> AIGPVADLTISNGAVSPDGFSRQAILVNDVFPSPLITGNKGDR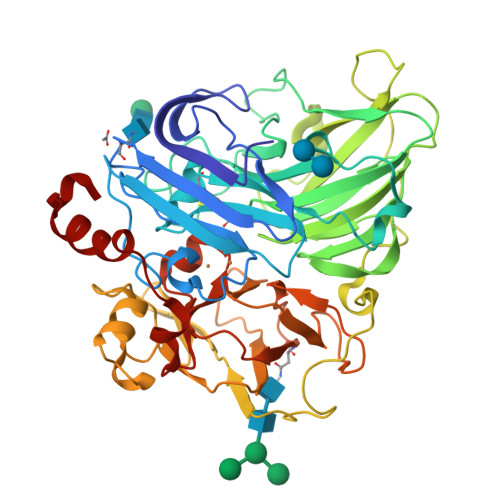FQLNVIDNMTNHTMLKSTSIHWHGFFQHGTNWADGPAFVNQCPISTGHAFLYDFQVPDQAGTFWYHSHLSTQYCDGLRGPIVVYDPNDPHKSLYDVDDDSTVITLADWYHLAAKVGAPVPTADATLINGLGRSSSTLAADLAVITVTKGKRYRFRLVSLSCDPNYTFSIDGHSLTVIEADSVNLKPHTVDSLQIFAAQRYSFVLNADQDVDNYWIRALPNSGTQNFAGGTNSAILRYDGAAPVEPTTSQTPSTNPLVESALTTLEGTAAPGSPTPGGVDLALNMAFGFAGGNFTINGASFTPPTVPVLLQILSGAQSAADLLPAGSVYSLPANADIEISLPATAAAPGFPHPFHLHGHIFAVVRSAGSSTYNYANPVYRDVVSTGAPGDNVTIRFRTDNPGPWFLHCHIDFHLEAGFAVVMAEDIPDVAATNPVPQAWSDLCPTYDALSPDDQ> SRLVEPYLDGYATSNVTTQIGTHAYLPCRVKQLGNKSVSWIRLRDGHILTVDRAVFIADQRFLAIKQPDKYWTLQIKYVQARDAGSYECQVSTEPKVSARVQLQVVVPHHHHHH;> SRLDPDPEFIGFINNVTYPAGREAILACSVRNLGKNKVGWLRASDQTVLALQGRVVTHNARISVMHQDMHTWKLKISKLRESDRGCYMCQINTSPMKKQVGCIDVQVPPDIINEESSADLAVQEGEDATLTCKATGNPQPRVTWRREDGEMILIRKPGSRELMKVESYNGSSLRLLRLERRQMGAYLCIASNDVPPAVSKRVSLSVHHHHHHH

We have recently identified interactions between two groups of Drosophila IgSF (immunoglobulin superfamily) cell adhesion molecules with properties closely matching a neuronal chemoaffinity function: 21 Dpr proteins, named after the founding member Defective proboscis extension response, selectively bind nine proteins, now called the Dpr-interacting proteins, or DIPs. All 21 Dprs and nine DIPs are predicted to contain two and three immunoglobulin (IG) domains, respectively. Our previous work identified the first IG domains, termed IG1, as the domains mediating the Dpr–DIP interaction by the formation of a pseudo-symmetric IG1-IG1 heterocomplex using the GFCC’C’ face of the immunoglobulin fold. Therefore, Dprs and DIPs are strong candidates for a synapse specification or targeting function.

We crystallized and solved the structures of Dpr1 IG1 with DIP-η IG1, and Dpr11 IG1 with DIP-γ IG1 +2. Interestingly, while the pairwise sequence identities among the three Dpr–DIP pairs are comparable (49% to 56%), the Dpr11–DIP-γ structure is significantly different than the other two. When the interface residues at the Dpr subunits are superimposed, the three DIP subunits are slightly displaced, with DIP-γ (dark gray in Figure 3) more distant from the other DIPs (~1.2 Å at the interface and up to 3 Å at the back face of the IG domain, Figure 3a; see Figure 3—figure supplement 1b for details of the displacement at the interface). Hence, different Dpr–DIP complexes can be established not only through shape complementarity between Dpr and DIP surfaces, but also by small but significant movements of the Dpr and DIP monomers with respect to each other, a mechanism not commonly recognized for related interaction pairs. A second highly variable position, Leu154 in Dpr11 (Lys in Dpr1 and His in Dpr6) also fails to explain specificity via simple electrostatic or hydrophobic matching (Figure 3d2): The interfacing residue in the three DIPs is a glutamine or lysine (Gln78 of DIP-γ), which is pushed away by the hydrophobic Leu154 of Dpr1, but not in complexes with Dpr6 or 11. This movement of Gln78 in DIP-γ is then accommodated by a glycine in Dpr11 position 157, which is otherwise a bulkier and hydrophobic Leu and Ile in Dpr1 and 6. Therefore, the Dpr11–DIP-γ crystal structure enables us to see that Leu154 and Gly157 in Dpr11 are structurally linked and are needed for DIP-γ binding. Interestingly, the position equivalent to Gly157 of Dpr11 (and Dpr15) in the two other DIP-γ binders, Dprs 16 and 17, are larger but polar amino acids (Figure 3d2), which can still be accommodated at the site as hydrogen bond participants with Q78 in DIP-γ. However, in Dpr11–DIP-γ, for which our structure unexpectedly shows no hydrogen bond, the His-to-Ala mutation abolished binding by more than five-fold. The A165Y mutation is expected to create of a hydrogen bond absent in the Dpr11–DIP-γ complex but present in Dpr6–DIP-α and the engineered Dpr11 A165Y F167Y K207V–DIP-α complex.AGDC1 and PPP2 fit in none of these categories as both enzymes neither display cofactors bound to their active sites nor require the styrene motif or ATP hydrolysis. Instead, they act on the carboxyl-group directly attached to the aromatic ring. Intriguingly, these enzymes’ catalytic mechanism is a new type of decarboxylation mechanism combining acid–base catalysis by a His-Asp dyad with a sophisticated web of hydrogen bonds and a double tryptophan twisting clamp. The trimers of AGDC1 and PPP2 in the crystal structures represent the functional biological unit, evidenced by the size exclusion chromatography data and the extensive intermonomer buried surfaces and interactions.

AGDC1 4NC/Co2+-complex had only one molecule in the AU in the space group P321, like the PPP2 crystal structures. The substrate binds in a deep cleft within the β-barrel. In the 4NC/Co2+ complex, the cobalt binding sites link the N-terminal regions of adjacent protomers. R39 anchors 4NC in the active site through an interaction with the negatively charged nitro-group, and the hydroxyl groups of 4NC form hydrogen bonds with Q192, T60, and Y150. H86 points to the si-face of the ligand and interacts with D40, forming a catalytic dyad. The nitro-group of 4NC is rotated by ~ 24° with respect to the catechol ring through interactions of the oxygen atoms with the nitrogen-hydrogens of two conserved tryptophan residues, W35 and W61, which create a tryptophan-clamp. The cobalt binding site in the crystal structure was identified by anomalous X-ray scattering. The cobalt ion is octahedrally coordinated by E49 and H14, each from a different monomer, located at the N-termini of neighboring chains, and four water molecules. To investigate the interactions between AGDC1 and its native substrate, we docked gallic acid into the active site of the 4NC/Co2+-complex structure using an induced fit procedure. Here, the gallate’s binding mode was virtually identical to that of 4NC. However, the additional hydroxyl-group present in gallate forms hydrogen-bonds with two more residues: Y146 and Y150, while Y146 does not interact with 4NC in the crystal structure.

> MTTSYEPWPQLYSHLNGTNEEVLDRMKVAELCKGWSVYRDASEWANFKEMFTPDANIWTTWSGAQTIDSFIQISKDGKDKGAFIMHRECGTLVDLNPKTQRAIGKMKTTITQRFEYEGVPFDIDCDNYFIFFCLKDSNGDWKARWYKVFYVKDKFVPVGVPTAENMEKLAKLFSKENLEQYPWGYQYLAVAQANLGYPIDKKLPTWKNELYHTMYDAMKEWMEGKEIDLHW>MAAPSPTTTAAAAAAATTHHRVLLPSARPRAAPSSLRLPLRAQPHAHAHAQRARLAAPVAAAAPAPAASTASPESPASGAVAGKPTVLVAEKLGAAGLALLREFANVDCSYGLSPEDLRAKISLCDALIVRSGTKVGRDVFEASGGRLRVVGRAGVGIDNVDLAAATEHGCLVVNAPTANTVAAAEHGIALLTAMARNIAQADASLKAGKWQRNKYVGVSLVGKTLAILGFGKVGSEVARRAKGLGMHVIAHDPYASADRARAIGVELVSMEEAMTTADFISLHMPLTPATDKMLNDEAFAKM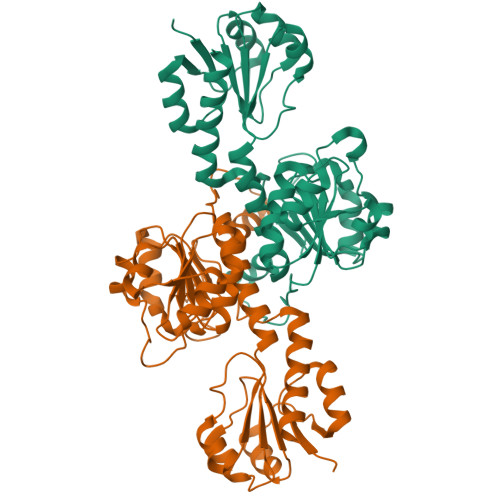KKGVRIINVARGGVIDEEALVRALDSGVVAQAALDVFTKEPPAADNKLVLHGNVTVTPHLGASTVEAQEGVAIEIAEAVIGALK[2x]>[12x]GLVPRGSHMGSMGIEYRSLHTSQLTLSEKEALY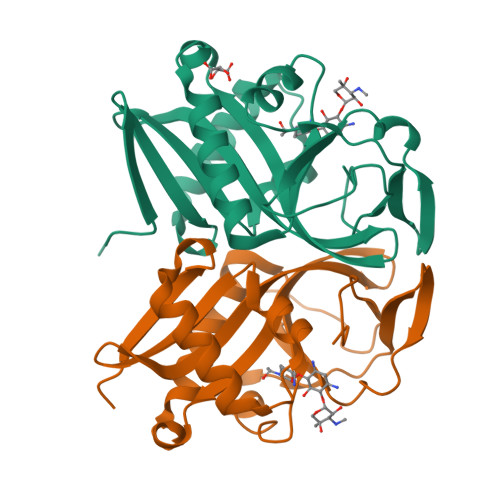DLLIEGFEGDFSHDDFAHTLGGMHVMAFDQQKLVGHVAIIQRHMALDNTPISVGYVEAMVVEQSYRRQGIGRQLMLQTNKIIASCYQLGLLSASDDGQKLYHSVGWQIWKGKLFELKQGSYIRSIEEEGGVMGWKADGEVDFTASLYCDFRGGDQW> MDFTKPETVLNLQNIRDELVRMEDSIIFKFIERSHFATCPSVYEANHPGLEIPNFKGSFLDWALSNLEIAHSRIRRFESPDETPFFPDKIQKSFLPSINYPQILAPYAPEVNYNDKIKKVYIEKIIPLISKRDGDDKNNFGSVATRDIECLQSLSRRIHFGKF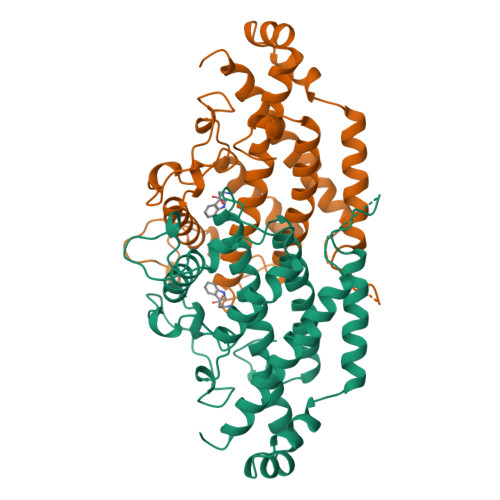VAEAKFQSDIPLYTKLIKSKDVEGIMKNITNSAVEEKILERLTKKAEVYGVDPTERRIERRISPEYLVKIYKEIVIPITKEVEVEYLLRRLEE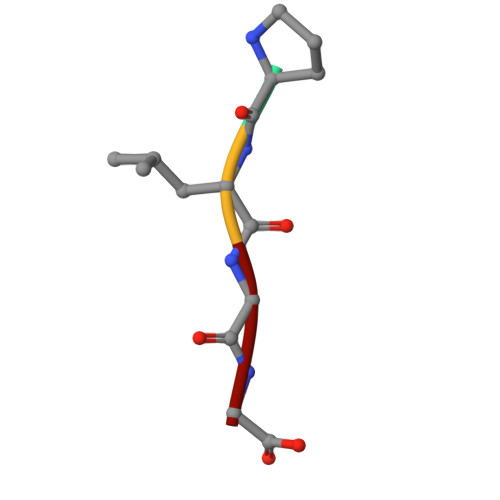> PLGG>MSFPYFISPEQAMRERSELARKGIARAKSVVALAYAGGVLFVAENPSRSLQKISELYDRVGFAAAGKFNEFDNLRRGGIQFADTRGYAYDRRDVTGRQLANVYAQTLGTIFTEQAKPYEVELCVAEVAHYGETKRPELYRITYDGSIADEPHFVVMGGTTEPIANALKESYAENASLTDALRIAVAALRAGSADTSGGDQPTLGVASLEVAVLDANRPRRAFRRITGSALQALLVDQESPQSDGESSG[14x];>ATIVALKYPGGVVMAGDRRSTQGNMISGRDVRKVYITDDYTATGIAGTAAVAVEFARLYAVELEHYEKLEGVPLTFAGKINRLAIMVRGNLAAAMQGLLALPLLAGYDIHASDPQSAGRIVSFDAAGGWNIEEEGYQAVGSGSLFAKSSMKKLYSQVTDGDSGLRVAVEALYDAADDDSATGGPDLVRGIFPTAVIIDADGAVDVPESR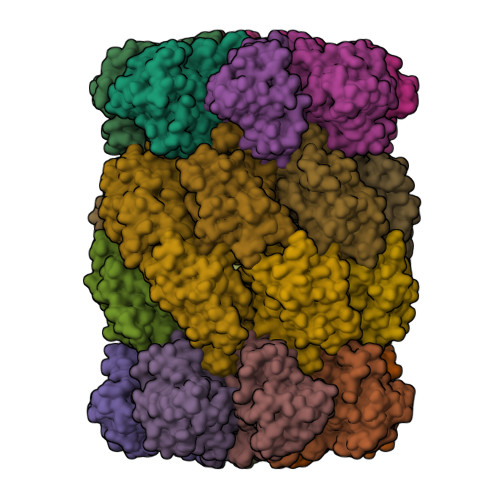IAELARAIIESRSGADTFGSDGGEK[14x]> DWVVAPISVPENGKGPFPQRLNQLKSNKDRDTKIFYSITGPGADSPPEGVFAVEKETGWLLLNKPLDREEIAKYELFGHAVSENGASVEDPMNISIIVTDLNDHKPKFTQDTFRGSVLEGVLPGTSVMQVTATDEDDAIYTYNGVVAYSIHSQEPKDPHDLMFTIHRS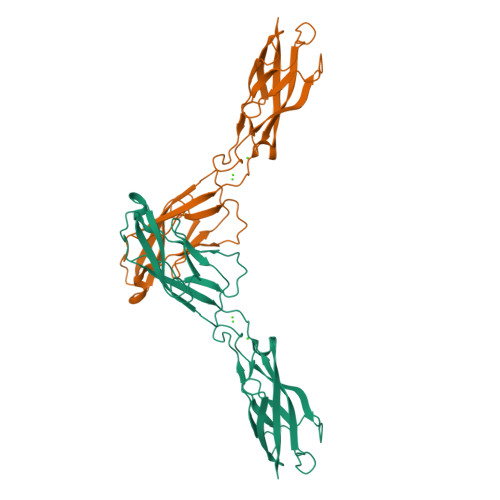TGTISVISSGLDREKVPEYTLTIQATDMDGDGSTTTAVAVVEILD> MEDLDERELKEAFRVLDKEKKGVIKVDVLRWILKSLGDELTEDEIENMIAETDTDGSGTVD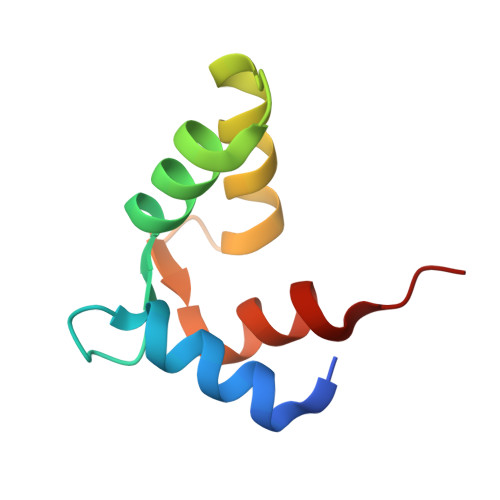YEEFKCLMMSSDA>MNRKWEAKLKQIEERASHYERKPLSSVYRPRLSKPEEPPSIWRLFHRQAQAFNFVKSCKEDVHVFALECKVG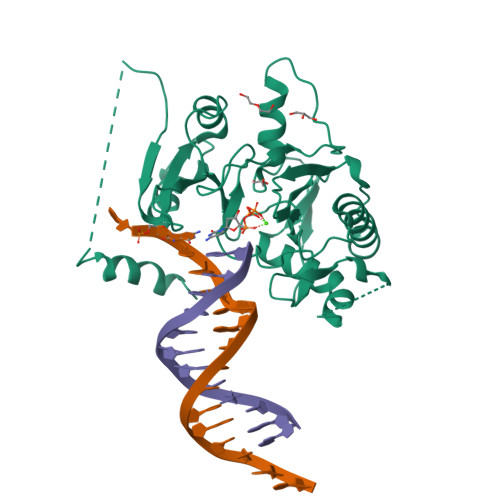DGQRIYLVTTYAEFWFYYKSRKNLLHCYEVIPENAVCKLYFDLEFNKPANPGADGKKMVALLIEYVCKALQELYGVNCSAEDVLNLDSSTDEKFSRHLIFQLHDVAFKDNIHVGNFLRKILQPALDLLGSEDDDSAPETTGHGFPHFSEAPARQGFSFNKMFTEKATEESWTSNSKKLERLGSAEQSSPDLSFLVVKNNMGEKHLFVDLGVYTRNRNFRLYKSSKIGKRVALEVTEDNKFFPIQSKDVSDEYQYFLSSLVSNVRFSDTLRILTCEPSQNKQK[2x]> MSGIALSRLAQERKAWRKDHPFGFVAVPTKNPDGTMNLMNWECAIPGKKGTPWEGGLFKLRMLFKDDYPSSPPKCKFEPPLFHPNVYPSGTVCLSILEEDKDWRPAITIKQILLGIQELLNEPNIQDPAQAEAYTIYCQNRVEYEKRVRAQAKKFAPS;> MGEGEYIKLKVIGQDSSEIHFKVKMTTHLKKLKESYCQRQGVPMNSLRFLFEGQRIADNHTPKELGMEEEDVIEVYQEQTGG;> SLNTGEPAPVLSSPPPADVSTFLAFPSPEKLLRLGPKSSVLIAQQTDTSDPEKVVSAFLKVSSVFKDEATVRMAVQDAVDALMQKAFNSSSFNSNTFLT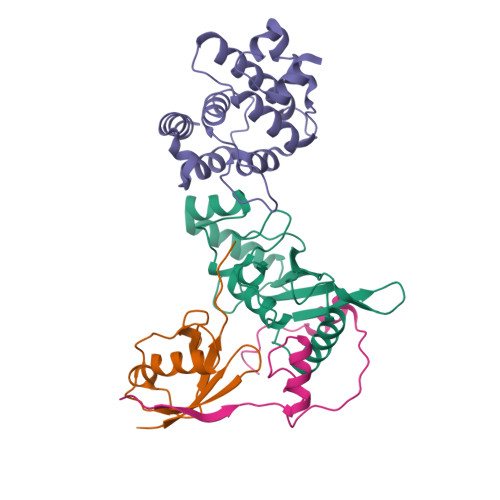RLLVHMGLLKSEDKVKAIANLYGPLMALNHMVQQDYFPKALAPLLLAFVTKPNSALESCSFARHSLLQTLYKV;> SLDVLIVYELTPTAEQKALATKLKLPPTFFCYKNRPDYVSEEEEDDEDFETAVKKLNGKLYLDGSEKCRPLEENTADNEKECI> MHHHHHHMIEELGKIDRIIQESVPGKQITLAHVIAAPIEAVYECLGVDHEGAIGVVSLTPNETAIIAADIAGDAANIDICFVD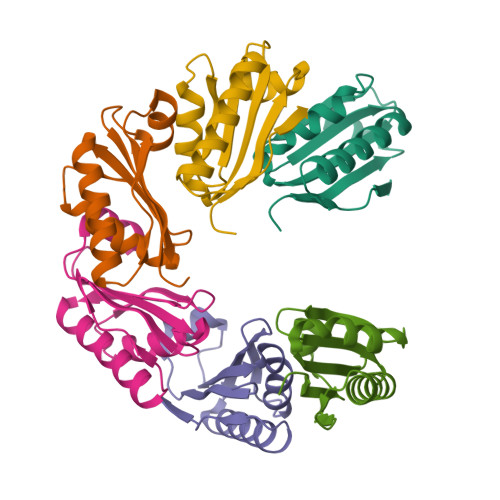RFTGSVMFSGDIQSVETSLEDILEYFKNSLGFSTVPLTKS>[20x]TLIELMIVVAIIGILAAIAIPQYQNYIAKSQVSRVMSETGSLKTVIETCILDGKTAANCELGWTNSNLLG;>[20x]STAAVTGQTGLTITYPASATESAAIQGTFGNSAAIKIKNQTLTWTRTPEGAWSCATTVEAKFKPAGCAS;> MNMYKWVPESIRDSGEGQPSYSNNGDYAPSGPWVAAGIHTMPQSLRDSMRNSIMVTAQARRDVIGPEWGPDGRFTGYASVIGTPDPKPADIVNKFTVERRPVSNGNFQQRVKAGDIVVAPYTSDGKITVKLVAGQKDISSTPDYDYRIDSSLASSAGFVVAGERWYYTKRHFIIPRYFQNWRMRRRKYVTGWVMPTFYSPKEIFNRLKDSLVPDTGLVTQVWADNNTKRMDFLTAMAEIPQTLSSFLDALGYLGSLIKDFKRRRFFLNKAHQRIRNKLGVSFAERRSQIVSKYDRKIASARKPAIIVKLRQRKEKALKALDKMRVREEKKMIREFATQAASLWLSFRYEIMPLYYQSQDVLDVIANSTSEFMTSRDFVAKAINIGIPLEWNLDQENLVSQPRHNVMVKSKLSPENNIGKTLSVNPFTTAWELLTLSFVVDWFVNFGDVIAGFTGGYSDDSGATASWRFDDKKVFHLKNIPSAMVIVDINFYTRQVIDPRLCGGLAFSPKLNLFRYLDAMSLSWNRSRLKISRAT

Single-stranded RNA bacteriophages (ssRNA phages) are positive-sense RNA viruses that have shown specificity for gram-negative bacteria by exploiting host retractile pili, including T4P6. Acinetobacters have type IV pili (T4P), which are involved in twitching motility, surface adhesion, biofilm formation, and natural transformation in gram-negative bacteria. Our study delves into the interaction between Acinetobacter phage AP205 and type IV pili. Using cryo-electron microscopy, we solve structures of the AP205 virion with an asymmetric dimer of maturation proteins, the native Acinetobacter type IV pili bearing a distinct post-translational pilin cleavage, and the pili-bound AP205 showing its maturation proteins adapted to pilin modifications, allowing each phage to bind to one or two pili.

To investigate the recognition mechanism between AP205 and T4P, we employed single-particle cryo-EM to obtain a structure of the AP205/T4P complex. The two copies of Mat exhibit different conformations: One Mat (referred as outer Mat) extends further to elevate its apical domain away from the capsid shell while the other Mat (referred as inner Mat) is embedded deeper within the capsid and has a larger bending angle between the central and basal domains. Within the T4P-Mat complex, the apical domain of each Mat specifically plugs into the groove formed by three adjacent pilin subunits within the T4P (referred to as Pilins 1, 2). Notably, the C-terminal Ser147 of Pilins 1 and 2 are positioned near β3 and β7 of the Mat apical domain, respectively. Apparently, glycosylation at these two serines can prevent binding of AP205 Mat. It is likely that the substoichiometric glycosylation of pilins allows AP205 to bind to unglycosylated sites on the T4P. We also observed that the internal cleavage site of Pilin 3 at Ser79 is located at the binding interface for the apical domain. This cleavage allows Ser79 to move ~13 Å away from Gly78, allowing its interaction with β8 of the Mat. The Mat of AP205 has evolved to adapt to such a post-translational cleavage at the phage-pilus binding interface and may not be compatible with an uncleaved pilin anymore.>[4x]MLSRKGIIPEEYVLTRLAEDPAEPRYRTRERRARFVSKKGNCNVAHKNIREQGRFLQDVFTTLVDLKWPHTLLIFTMSFLCSWLLFAMVWWLIAFAHGDLAPGEGTNVPCVTSIHSFSSAFLFSIEVQVTIGFGGRMVTEECPLAILILIVQNIVGLMINAIMLGCIFMKTAQAHRRAETLIFSKHAVITLRHGRLCFMLRVGDLRKSMIISATIHMQVVRKTTSPEGEVVPLHQVDIPMENGVGGNGIFLVAPLIIYHVIDSNSPLYDLAPSDLHHHQDLEIIVILEGVVETTGITTQARTSYLADEILWGQRFVPIVAEEDGRYSVDYSKFGNTIKVPTPLCTARQLDEDRSLLDALTLASSRGPLRKRSVAVAKAKPKFSISPDSLS;>[4x]MPLAFCGTENHSAAYRVDQGVLNNGCFVDALNVVPHV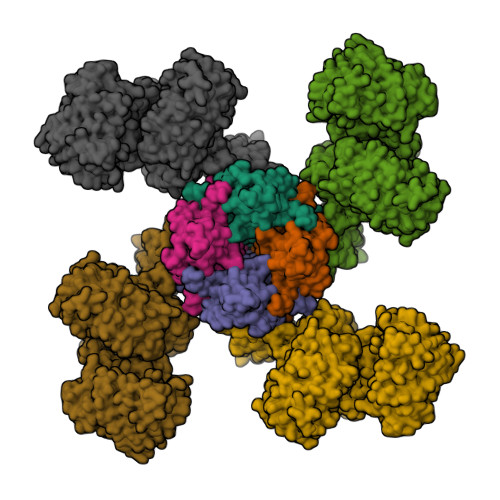FLLFITFPILFIGWGSQSSKVHIHHSTWLHFPGHNLRWILTFILLFVLVCEIAEGILSDGVTESRHLHLYMPAGMAFMAAITSVVYYHNIETSNFPKLLIALLIYWTLAFITKTIKFVKFYDHAIGFSQLRFCLTGLLVILYGMLLLVEVNVIRVRRYIFFKTPREVKPPEDLQDLGVRFLQPFVNLLSKGTYWWMNAFIKTAHKKPIDLRAIGKLPIAMRALTNYQRLCVAFDAQARKDTQSPQGARAIWRALCHAFGRRLILSSTFRILADLLGFAGPLCIFGIVDHLGKENHVFQPKTQFLGVYFVSSQEFLGNAYVLAVLLFLALLLQRTFLQASYYVAIETGINLRGAIQTKIYNKIMHLSTSNLSMGEMTAGQICNLVAIDTNQLMWFFFLCPNLWAMPVQIIVGVILLYYILGVSALIGAAVIILLAPVQYFVATKLSQAQRSTLEHSNERLKQTNEMLRGMKLLKLYAWESIFCSRVEVTRRKEMTSLRAFAVYTSISIFMNTAIPIAAVLITFVGHVSFFKESDLSPSVAFASLSLFHILVTPLFLLSSVVRSTVKALVSVQKLSEFLSSAEIREEQCAPREPAPQGQAGKYQAVPLKVVNRKRPAREEVRDLLGPLQRLAPSMDGDADNFCVQIIGGFFTWTPDGIPTLSNITIRIPRGQLTMIVGQVGCGKSSLLLATLGEMQKVSGAVFWNSNLPDSEGEDPSSPERETAAGSDIRSRGPVAYASQKPWLLNATVEENITFESPFNKQRYKMVIEACSLQPDIDILPHGDQTQIGERGINLSGGQRQRISVARALYQQTNVVFLDDPFSALDVHLSDHLMQAGILELLRDDKRTVVLVTHKLQYLPHADWIIAMKDGTIQREGTLKDFQRSECQLFEHWKTLMNRQDQELEKETVMERKASEPSQGLPRAMSSRDGLLLDEEEEEEEAAESEEDDNLSSVLHQRAKIPWRACTKYLSSAGILLLSLLVFSQLLKHMVLVAIDYWLAKWTDSALVLSPAARNCSLSQECDLDQSVYAMVFTLLCSLGIVLCLVTSVTVEWTGLKVAKRLHRSLLNRIILAPMRFFETTPLGSILNRFSSDCNTIDQHIPSTLECLSRSTLLCVSALTVISYVTPVFLVALLPLAVVCYFIQKYFRVASRDLQQLDDTTQLPLLSHFAETVEGLTTIRAFRYEARFQQKLLEYTDSNNIASLFLTAANRWLEVRMEYIGACVVLIAAATSISNSLHRELSAGLVGLGLTYALMVSNYLNWMVRNLADMEIQLGAVKRIHALLKTEAESYEGLLAPSLIPKNWPDQGKIQIQNLSVRYDSSLKPVLKHVNALISPGQKIGICGRTGSGKSSFSLAFFRMVDMFEGRIIIDGIDIAKLPLHTLRSRLSIILQDPVLFSGTIRFNLDPEKKCSDSTLWEALEIAQLKLVVKALPGGLDAIITEGGENFSQGQRQLFCLARAFVRKTSIFIMDEATASIDMATENILQKVVMTAFADRTVVTIAHRVHTILSADLVMVLKRGAILEFDKPETLLSQKDSVFASFVRADK(2S)-2-AMINO-4-[METHYL(PHOSPHONOOXY)PHOSPHORYL]BUTANOIC 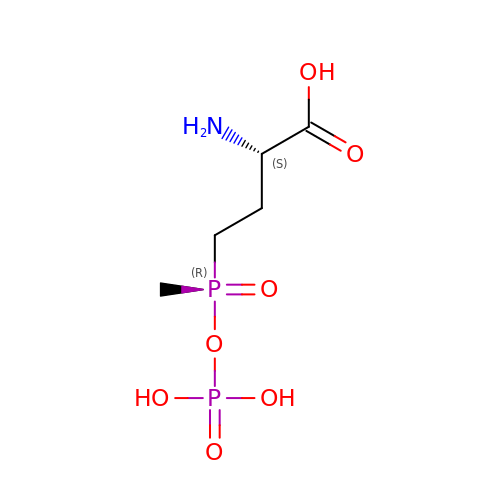ACID | C5 H13 N O7 P2 | UXRZHSKRCMUNIN-YZSVAWROSA-N> IVGGYTCAANSIPYQVSLNSGSHFCGGSLINSQWVVSAAHCYKSRIQVRLGEHNIDVLEGNEQFINAAKIITH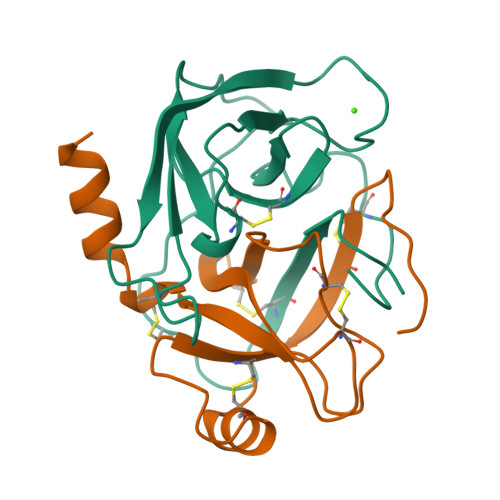PNFNGNTLDNDIMLIKLSSPATLNSRVATVSLPRSCAAAGTECLISGWGNTK;> SSGSSYPSLLQCLKAPVLSNSSCKSSYPGQITGNMICVGFLQGGKDSCQGDSGGPVVCNGQLQGIVSWGYGCAQKNKPGVYTKVCNYVNWIQQTIAAN> MLLLARCLLLVLVSSLLVCSGLACGPGRGFGKRRHPKKLTPLAYKQFIPNVAEKTLGASGRYEGKISRNSERFKELTPNYNPDIIFKDEENTGADRLMTQRCKDKLNALAISVMNQWPGVKLRVTEGWDEDGHHSEESLHYEGRAVDITTSDRDRSKYGMLARLAVEAGFDWVYYESKAHIHCSVKAENSVAAKSGGCFPGSATVHLEQGGTKLVKDLSPGDRVLAADDQGRLLYSDFLTFLDRDDGAKKVFYVIETREPRERLLLTAAHLLFVAPHNDSATGEPEASSGSGPPSGGALGPRALFASRVRPGQRVYVVAERDGDRRLLPAAVHS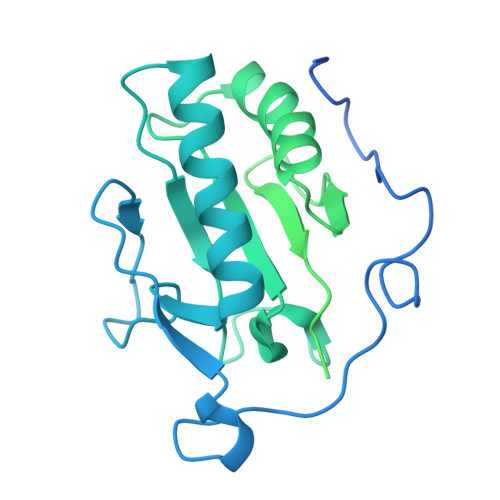VTLSEEAAGAYAPLTAQGTILINRVLASCYAVIEEHSWAHRAFAPFRLAHALLAALAPARTDRGGDSGGGDRGGGGGRVALTAPGAADAPGAGATAGIHWYSQLLYQIGTWLLDSEALHPLGMAVKSS>[2x]MGCSEKININEDKISHKIDIPDSAWTIGIGEKFKNAGHPNVKYPMIDDSYVQGAPLGGFGAGTIGRTYNGGFSRWHLEIGKNKYTTVYANQFSVFQKVEGNKDGVAQVLYAGEPENGYLSSWKWDYPKESGMYYALYPNSWYTYTNKDLPVQLAVKQFSPIIPYNYKETSYPVAVFKWTAYNPTNKNVDVSIMFTWQNMIGFFGKQVNVNSGNFNKIIKDKSKDSEIVAAVMGNISNDNEEWNGEYSIGVKKVPGVDISYKAKFVTTGDGSDLWHEFSKNGILDNKDDETPTKQDGIGSAIAVNFKLQPGQTIEVPFALSWDLPIMKFGGGDKWYKMYTKYFGKNGKNSFAILKEALNNYQKWEKMIDDWQKPILSNKSKPDWYKTALFNELYYLADGGTAWENGKVGEKDKRTNNMFGLLECFDYNYYETLDVRFYGSFPLVMLWPDIEKQVMRQFADTINVQDSSEFKVGSNGAMAV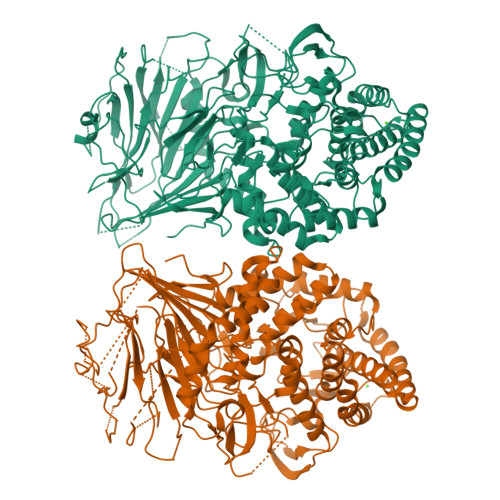KKVQGMIPHDLGSSYALPWIKINAYDWQNPNIWKDLNSKYVLLVYRDYVLTGKTDKEFLKYTWKSVKTALDKLKEMDKDNDGIPDNEGIPDQTYDTWSMKGTSAYCGSLWLAALKAAQEIGKVLKDNEAYIKYNEWYKIAQQNFEKELWNGEYYNFDTESDHKDSIMADQLAGQWYADILRLGDILPKDHVQKALKKIYEFNVMKFENGKMGAVNGMRPDGIVDESDIQAQEVWTGVTYALASFMKYRGMTEEAYNTAYGVYKMTYDKSGKGYWFRTPEAWTKDGNYRASMYMRPLSIWSMEVNYNEV> TFTSDSASTRFSQAFGIQTGDAVASTITVFQALSIDDQLAVLWYAYTEMGRS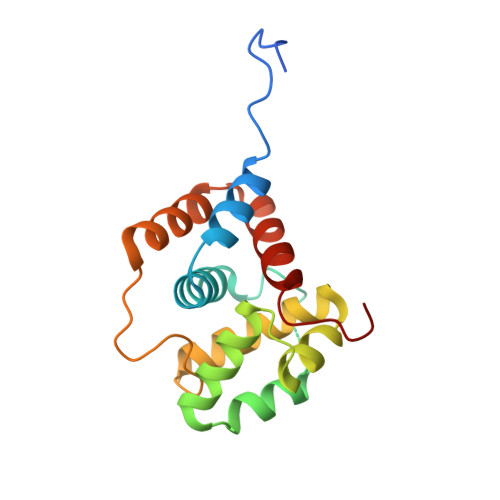ITPAATGAARLQLAEGLLNQIKQMSHAEQLQVMRDLAAKNNTQVSRSYGILSNNTKLAFWYELSELMVKGFVVPVPTDYKISRDGSQVLEALKGLDFCQQITVLRKVVADMGVDPLA(6~{R})-3-methyl-8-[(2~{S},4~{R},5~{S},6~{R})-6-methyl-5-[(2~{S},4~{R},5~{R},6~{R})-6-methyl-4-[(2~{S},5~{S},6~{S})-6-methyl-5-[(2~{S},4~{R},5~{S},6~{R})-6-methyl-5-[(2~{S},4~{S},5~{S},6~{R})-6-methyl-4-[(2~{S},5~{S},6~{S})-6-methyl-5-oxidanyl-oxan-2-yl]oxy-5-oxidanyl-oxan-2-yl]oxy-4-oxidanyl-oxan-2-yl]oxy-oxan-2-yl]oxy-5-oxidanyl-oxan-2-yl]oxy-4-oxidanyl-oxan-2-yl]oxy-1,6,11-tris(oxidanyl)-5,6-dihydrobenzo[a]anthracene-7,12-dione 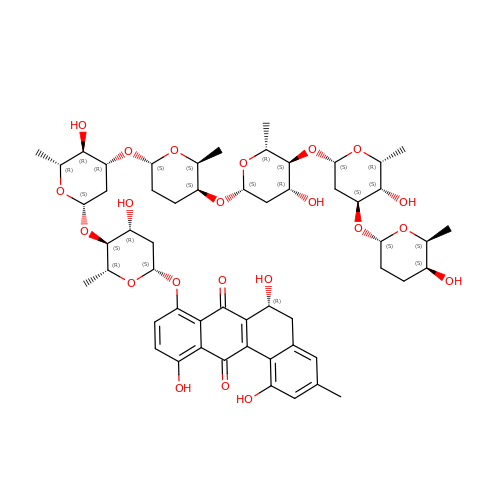| C55 H74 O22 | YMSZNAXJMXNNPT-HUUHVTJASA-N> TETTSFSITKFGPDQQNLIFQGDGYTTKERLTLTKAVRNTVGRALYSSPIHIWDSKTGNVANFVTSFTFVIDAPNSYNVADGFTFFIAPVDTKPQTGGGYLGVFNSKDYDKTSQTVAVEFDTFYNTAWDPSNGDRHIGIDVNSIKSINTKSWALQNGKEANVVIAFNAATNVLT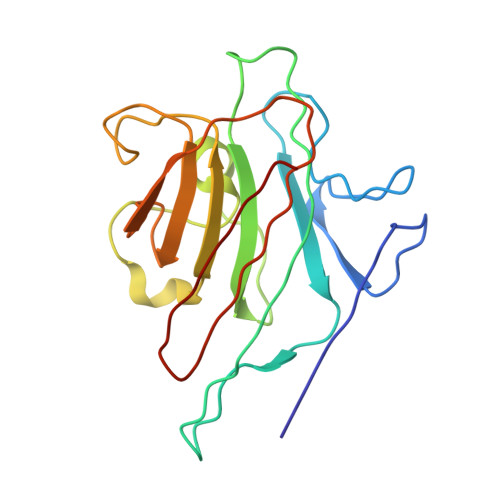VSLTYPN NadR converts NR into nicotinamide mononucleotide (NMN) and subsequently into NAD. Here, we report the first structural and biochemical characterization of a NadR protein from a Gram-positive bacterium (Lactococcus lactis), and compare it with the Gram-negative ortholog. Each molecule of NadRLl is comprised of two domains—an N-terminal NMNAT domain (residues 8–177) folded in a Rossmann-like fold and a C-terminal RNK domain (residues 178–379). While NadR proteins from Haemophilus sp. and most Gram-negative bacteria contain a DNA binding domain at the N terminus, such a domain is absent in the NadRLl protein, indicating that NadRLl is not involved in transcriptional regulation.

NadRLl crystallized in the P6422 space group with two molecules in the asymmetric unit. In the previously reported NadRHi crystal structure, NAD was bound to the NMNAT domain; however, we did not observe NAD molecules bound to the NMNAT domain of NadRLl. Interestingly, we observed strong positive electron density in the region between the two domains whenever we added substrates for co-crystallization. In one of the collected datasets, we observed a mixture of NAD and AMP-PNP bound at this location in the electron density. Additionally, we obtained structures in the presence of NMN and NR, which both have bound substrates in a similar area. This novel ‘binding site’ is very different from the canonical binding sites in NMNAT and RNK domains and is formed by side chains of K65, Y69, R177, H178, Y240, S244, N248, and R293. Here we observed electron density for an NAD or other nucleotide molecule at a different site, located between the two domains, whereas the predicted active sites were unoccupied. Although we cannot completely rule out that the new binding site is an artifact of crystallization, another explanation is that this site is a transfer hub between two domains. The site may also have a function for allosteric regulation, which could explain the sigmoidal dependence of the conversion of NMN to NAD on the ATP concentration. The measured binding affinities for Mg2+-complexed ATP and AMP-PNP are 63 µM and 13 µM, respectively.

>[2x]MLTNNISKSKLSGKNIGIYFGTFAPLHTGHQQQIYKCASLNDGVLLVVSGYDNDRGAQIGLPLEKRFRYLREAFNDEENIKVSMLNENDLPEMPNGWDEWANRLFELIHHNTLENDLSVTFYVGELEYAAELKKRFPADGNQYAVEIADRHDISLSATQIRENPQEHWTHINRVFRRHFSKVVTVMGSASTGKTTLVRRLARSINAPFSEEYAREYEEAFNIDDDELKMDDYARMITGQYDANSREVNSPANQGIVFLDTDAIVTRVYAKLYLPKEDFEQLEPLFRKTIADERMDLILVIPPITEYIDDGFRHMEWEESRHEFHEELMRQLAEFGLLDKVVILDDEGDHRDQEGYLTRYHHAIDAVHEYTGVKIERLSY[[N-(BENZYLOXYCARBONYL)AMINO]METHYL]PHOSPHATE | C9 H12 N O5 P | 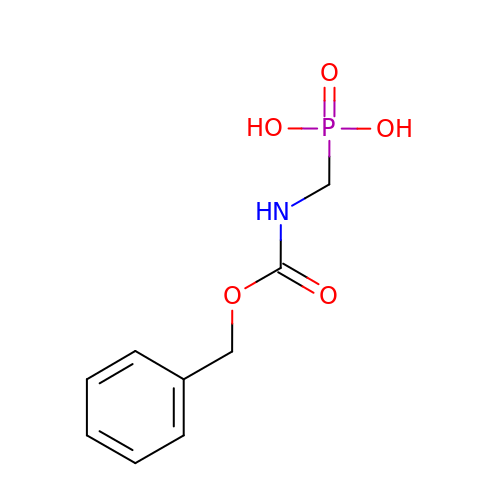WUNKRZNFNIYEPN-UHFFFAOYSA-N>[2x]MGHHHHHHSSGLVPRGSATERQDRNLLYEHAREGYSALPLLDMESLCAYPEDAARALDLRKGELRS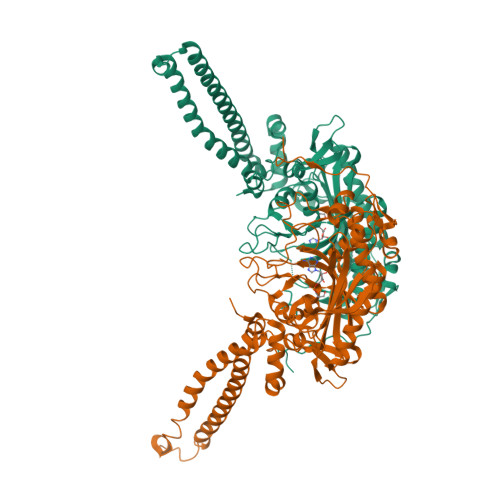KDLPGIISTWQELRQLREQIRSLEEEKEAVTEAVRALVVNQDNSQVQQDPQYQSLRARGREIRKQLTLLYPKEAQLEEQFYLRALRLPNQTHPDVPVGDESQARVLHVVGDKPAFSFQPRGHLEIAEKLDIIRQKRLSHVSGHRSYYLRGAGALLQHGLVNFTLNKLIHRGFTPMTVPDLLRGVVFEGCGMTPNAKPSQIYNIDPSRFEDLNLAGTAEVGLAGYFMDHSVAFRDLPIRMVCSSTCYRAETDTGKEPWGLYRVHHFTKVEMFGVTGPGLEQSSELLEEFLSLQMEILTELGLHFRVLDMPTQELGLPAYRKFDIEAWMPGRGRFGEVTSASNCTDFQSRRLHIMFQTEAGELQFAHTVNATGCAVPRLLIALLESYQQKDGSVLVPPALQPYLGTDRITTPTHVPLQYIGPNQPQKPRLPGQPASS>SDVRPPHILVKTLDYIVDNLLTTLPESEGFLWDRMRSIRQDFTYQNYSGPEAVDCNERIVRIHLLILHIMVKSNVEFSLQQELEQLH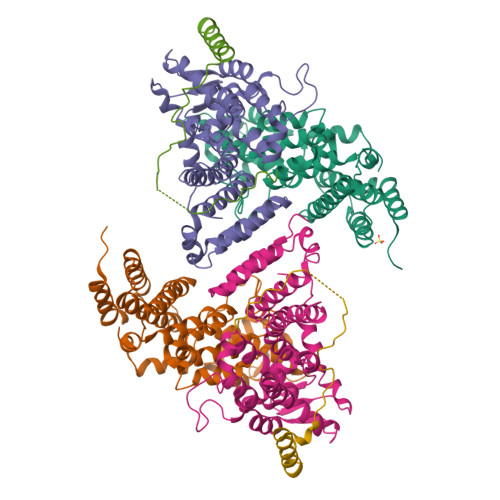KSLITLSEIYDDVRSSGGTCPNEAEFRAYALLSKIRDPQYDENIQRLPKHIFQDKLVQMALCFRRVISNSAYTERGFVKTENCLNFYARFFQLMQSPSLPLLMGFFLQMHLTDIRFYALRALSHTLNKKHKPIPFIYLENMLLFNNRQEIIEFCNYYSIEIINGDAADLKTLQHYSHKLSETQPLKKTYLTCLERRLQKTTYKGLINGGEDN[2x];>[2x]GKQRILLYLVNKLNNIYFRIESPQLCSNIFKNFQPKSMLAHFNEYQLDQQIEYRYLLGRYYLLNSQVHNAFVQFNEAFQSLLNLPLTNQAITRNGTRILNYMIPTGLILGKMVKWGPLRPFLSQETIDNWSVLYKHVRYGNIQGVSLWLRQNERHLCARQLLIVLLEKLPMVTYRNLIKTVIKSWTTEWGQNKLPYSLIERVLQLSIGPTFEDPGAQEITIYNGIHSPKNVENVLVTLINLGLLRANCFPQLQLCVVKKTTMIQEIVPPVNERITKMFPAHSHVLW;>[2x]EEDDEFEDFPIDTWANGETIKSNAVTQTNIWEENWDDVEVDDDFTNELKAELDRYKRENQ> AAQLSEQLAELEKRSGGRLGVAVLDTATGRRIAYRGDERFPMCSTFKALLAAAVLARVDQGKERLDRRITYGKEDLVDYSPVTEKHVGDGMTVAELCEAAITLSDNTAANLLLEALGGPAALTAFLRSIGDEVTRLDRWEPELNEAAPGDPRDTTTPAAMAATLRTLLLGDALSPASRQQLVDWLVANKTGDKRLRAGLPADWRVGDKTGTGGHGTTNDIAVIWPPGRAPIVVTVYLTESQV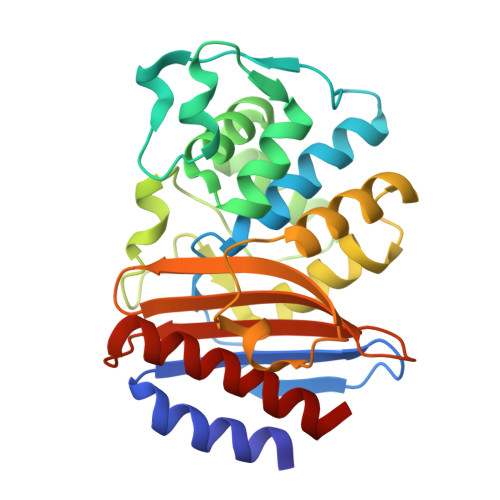DADARDAVIAEVGRLVVEAF> PAGRSIYNSFYVYCKGPCQRVQPGKLRVQCSTCRQATLTLTQGPSCWDDVLIPNRMSGECQSPHCPGTSAEFFFKCGAHPTSDKETSVALHLIATNSRNITCITCTDVRSPVLVFQCNSRHVICLDCFHLYCVTRLNDR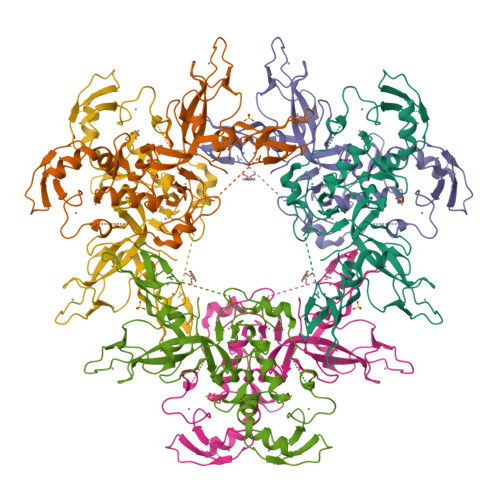QFVHDPQLGYSLPCVAGCPNSLIKELHHFRILGEEQYNRYQQYGAEECVLQMGGVLCPRPGCGAGLLPEPDQRKVTCEGGNGLGCGFAFCRECKEAYHEGECSAVFEASGTTTQAYRVDERAAEQARWEAASKETIKKTTKPCPRCHVPVEKNGGCMHMKCPQPQCRLEWCWNCGCEWNRVCMGDHWFDV> ASMLEAKFEEASLFKRIIDGFKDCVQLVNFQCKEDGIIAQAVDDSRVLLVSLEIGVEAFQEYRCDHPVTLGMDLTSLSKILRCGNNTDTLTLIADNTPDSIILLFEDTKKDRIAEYSLKLMDIDADFLKIEELQYDSTLSLPSSEFSKIVRDLSQLSDSINIMITKETIKFVADGDIGSGS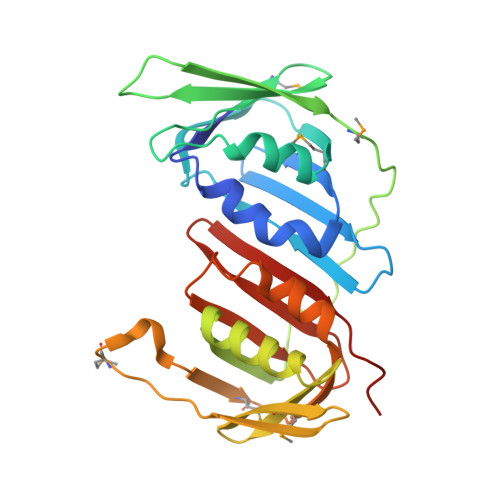VIIKPFVDMEHPETSIKLEMDQPVDLTFGAKYLLDIIKGSSLSDRVGIRLSSEAPALFQFDLKSGFLQFFLAPKFNDEE In this study, we identified and characterized a typhoid toxin-like A2B5 toxin, designated diarizonae toxin (DiaT), as a key virulence factor in Salmonella diarizonae. The DiaT genomic islet encodes two distinct B subunits, PltBd1 and PltBd2, which exhibit unique functional roles. Through genetic and functional analyses, we demonstrate that the heteropentameric assembly of PltBd1 and PltBd2 is essential for cytotoxicity, with our data suggesting PltBd1 facilitates toxin secretion and PltBd2 mediates host cell targeting. The holotoxin consists of a pentameric B subunit arrangement supporting a single PltA subunit, with the amphipathic C-terminal tail of PltA extending into the central pore formed by the B subunits.

To elucidate the structural assembly of PltBd1 and PltBd2 within the DiaT holotoxin, we introduced a C-terminal Strep-tag on CdtB in the S. diarizonae genome. DiaT was purified from cultures grown in TTIM medium using Strep-Tactin affinity purification and gel filtration, followed by cryo-EM analysis. Ultimately, we obtained only a single class of high-resolution cryo-EM map for the holotoxin, at a resolution of 2.32 Å. Despite clear visualization of CdtB in 2D classifications, its flexible linkage to PltA, mainly via a single disulfide bond, caused a weakened signal, leading to its absence in the final 3D reconstruction. To distinguish PltBd1 from PltBd2 in the cryo-EM map, we identified residues with distinct structural features between PltBd1 and PltBd2. Specifically, Ile25 and Tyr82 in PltBd1 corresponded to Phe24 and Val80 in PltBd2, respectively, providing clear markers for differentiation. Detailed analysis of electron density maps revealed a pseudo-symmetric arrangement of the pentameric B subunits, comprising a 3:2 ratio of PltBd1 to PltBd2. Three tightly packed PltBd1 subunits were connected with dimeric PltBd2 subunits to form the heteropentamer in the holotoxin structure. Pore radius measurements confirmed that the PltBd1 homopentamer exhibits the smallest pore radius with significant distortion, while the PltBd2 homopentamer displays a larger and straighter pore. These findings suggest that the specific positioning of Tyr70 in PltBd1 is responsible for the pore contraction in the heteropentamer, which enhances compatibility with the C-terminal tail of PltA. The stronger hydrophobic interactions between PltBd2 and PltA, along with additional polar interactions involving PltBd1 and PltA, establish a finely balanced assembly that facilitates the stable accommodation of PltA’s C-terminal tail by the heteropentameric B subunits.

> IDFVYRVDPNPPDVIFRDGFSLLGYNRDLQQLISGRSCAGGSSDSRYIVTTSDINKTYAIARAYYSHSKFKGNLYRYKIRADNNFYSLTPSVNYLESQGGHFNAYEKSMIRLQSEYVSTLSILPENIQKAVALVYDSSTGQIKDGTSTINTDYVSISSVSNPGVIPFLPEPQANTQQRIDAFGSLISSCFSIYSVCQTHRGQKTEVYKMPFYDARPVIQFIISGN;>[3x]EWTGDYENIGYFSHEVISEFHVGQIDGGAYFCIKAVKADGSRSTPLIACSVSNESVWAPSFKVLLEQARYFYVTEQSVRIYYDHNVWTNQPFVNTFSTNALVGLSSCSAATDCFGPGKP;>EWTGDSSINYYSDEVISDFHVGQFNRSAYFCIKTVKKSGEGTPIIACALSHDSKWIPSFNIMLEQARNFYITGHSIRVYVQPNVWSNKSFIEALSSNALVGLSSCSTSECFGPVK[2x]6-(2-{3-[3-(dimethylamino)propyl]-2,5-difluorophenyl}ethyl)-4-methylpyridin-2-amine 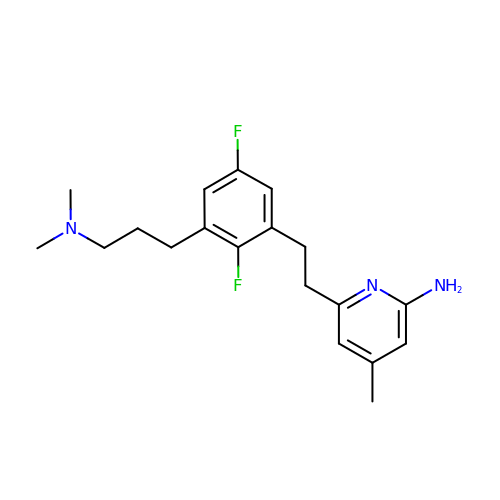| C19 H25 F2 N3 | ZUJBVDNPPNRQBW-UHFFFAOYSA-N> GSHPLGDTSDASKLSSDYSLPDLINTRKVPNNWQTGEQASLEEGRIVLTSNQNSKGSLWLKQGFDLKDSFTMEWTFRSVGYSGQTDGGISFWFVQDSNIPRDKQLYNGPVNYDGLQLLVDNNGPLGPTLRGQLNDGQKPVDKTKIYDQSFASCLMGYQDSSVPSTIRVTYDLEDDNLLKVQVDNKVCFQTRKVRFPSGSYRIGVTAQNGAVNNNAESFEIFKMQFFNGVIEDSLIPNVNAMG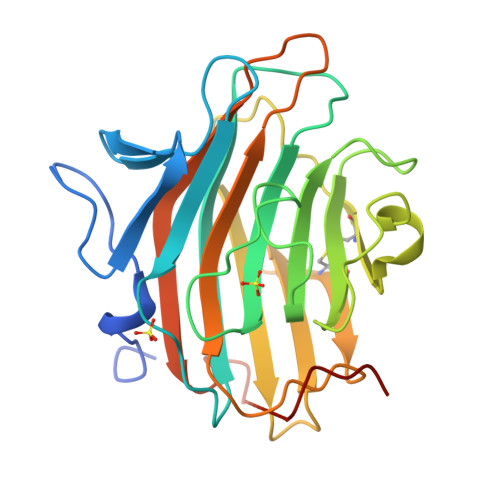QPKLITKYIDQQTG>[6x]MSGPKKYFPIPVEHLEEEIRIRSADDCKQFREEFNSLPSGHIQGTFELANKEENREKNRYPNILPNDHSRVILSQLDGIPCSDYINASYIDGYKEKNKFIAAQGPKQETVNDFWRMVWEQKSATIVMLTNLKERKEEKCHQYWPDQGCWTYGNIRVCVEDCVVLVDYTIRKFCIQPQLPDGCKAPRLVSQLHFTSWPDFGVPFTPIGMLKFLKKVKTLNPVHAGPIVVHCSAGVGRTGTFIVIDAMMAMMHAEQKVDVFEFVSRIRNQRPQMVQTDMQYTFIYQALLEYYLYGDTELDVSSLEKHLQTMHGTTTHFDKIGLEE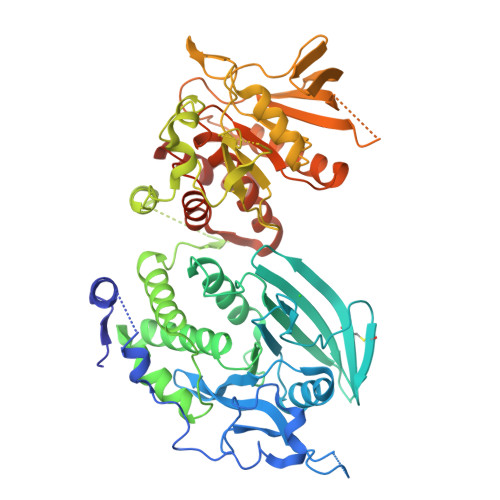EFRKLTNVRIMKENMRTGNLPANMKKARVIQIIPYDFNRVILSMKRGQEYTDYINASFIDGYRQKDYFIATQGPLAHTVEDFWRMIWEWKSHTIVMLTEVQEREQDKCYQYWPTEGSVTHGEITIEIKNDTLSEAISIRDFLVTLNQPQARQGEQVRVVRQFHFHGWPEIGIPAEGKGMIDLIAAVQKQQQQTGNHPITVHCSAGAGRTGTFIALSNILERVKAEGLLDVFQAVKSLRLQRPHMVQTLEQYEFCYKVVQDFIDIFSDYAAHHHHHH> MLPFLLATLGTTALNNSNPKDYCYSARIRSTVLQGLPFGGVPTVLALDFMCFLALLFLFSILRKVAWDYGRLALVTDADRLRRQERDRVEQEYVASAMH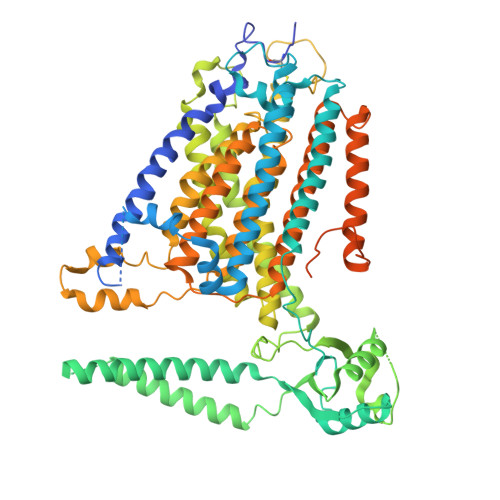GDSHDRYERLTSVSSSVDFDQRDNGFCSWLTAIFRIKDDEIRDKCGGDAVHYLSFQRHIIGLLVVVGVLSVGIVLPVNFSGDLLENNAYSFGRTTIANLKSGNNLLWLHTSFAFLYLLLTVYSMRRHTSKMRYKEDDLVKRTLFINGISKYAESEKIKKHFEEAYPNCTVLEARPCYNVARLMFLDAERKKAERGKLYFTNLQSKENVPTMINPKPCGHLCCCVVRGCEQVEAIEYYTKLEQKLKEDYKREKEKVNEKPLGMAFVTFHNETITAIILKDFNVCKCQGCTCRGEPRPSSCSESLHISNWTVSYAPDPQNIYWEHLSIRGFIWWLRCLVINVVLFILLFFLTTPAIIITTMDKFNVTKPVEYLNNPIITQFFPTLLLWCFSALLPTIVYYSAFFEAHWTRSGENRTTMHKCYTFLIFMVLLLPSLGLSSLDLFFRWLFDKKFLAEAAIRFECVFLPDNGAFFVNYVIASAFIGNAMDLLRIPGLLMYMIRLCLARSAAERRNVKRHQAYEFQFGAAYAWMMCVFTVVMTYSITCPIIVPFGLMYMLLKHLVDRYNLYYAYLPAKLDKKIHSGAVNQVVAAPILCLFWLLFFSTMRTGFLAPTSMFTFVVLVITIVICLCHVCFGHFKYLSAHNYKIEHTETDTVDPRSNGRPPTAAAVPKSAKYIAQVLQDSEVDGDGDGAPGSSGDEPPSSSSQDEELLMPPDALTDTDFQSCEDSLIENEIHQTRLEVLFQ>[2x]SNART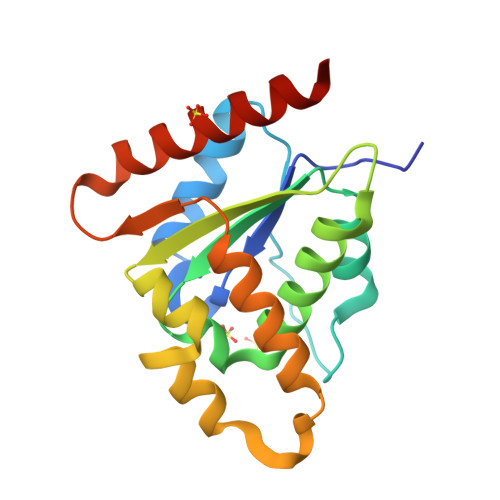ITYDVFLSFRGEDTRFNFTDHLYSALGRRGIRTFRDDKLRRGEAIAPELLKAIEESRSSVIVFSENYARSRWCLDELVKIMECHKDKKDPGHAVFPIFYHVDPSHVRKQEGSFGEAFAGYGENLKDKIPRWRTALTEAANLSGWPLQDGYESNQIKEITDSIFRRLKCKRLDAG> GAGCAGACCAG;> ACGTCACTCA;> CTCGT;> TCTGAGT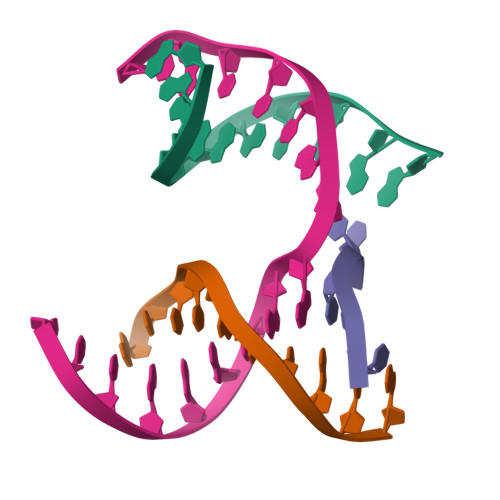GAGGTCTGC> GSHMKYTNPRFYKHPLFKNFNVTESENYLRSSTDDFLIRKGSRHGYCVLV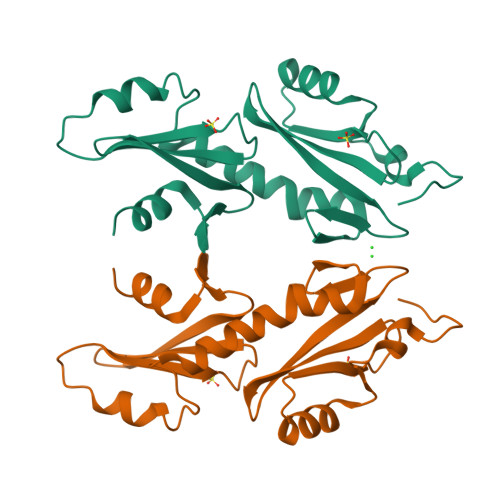IKFASDVFVHMKIEEHSEHYTCSNKHFEDIDEVISVYVRPILRNLKSIKAHAKYFNSPEDAEKLLSSFDGSKVVYAFYFSRKYPGKLTFAYNNGSILEEYIGVSDMLTYNNSTFKDIDSFVAYRKRLK> MALSTATKAATDALAANRAPTSVNAQEVHRWLQSFN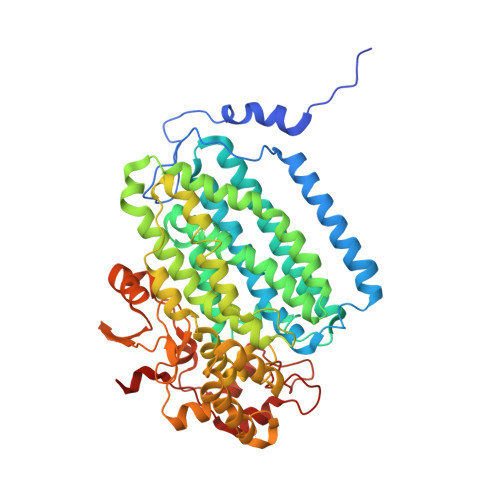WDFKNNRTKYATKYKMANETKEQFKLIAKEYARMEAVKDERQFGSLQDALTRLNAGVRVHPKWNETMKVVSNFLEVGEYNAIAATGMLWDSAQAAEQKNGYLAQVLDEIRHTHQCAYVNYYFAKNGQDPAGHNDARRTRTIGPLWKGMKRVFSDGFISGDAVECSLNLQLVGEACFTNPLIVAVTEWAAANGDEITPTVFLSIETDELRHMANGYQTVVSIANDPASAKYLNTDLNNAFWTQQKYFTPVLGMLFEYGSKFKVEPWVKTWNRWVYEDWGGIWIGRLGKYGVESPRSLKDAKQDAYWAHHDLYLLAYALWPTGFFRLALPDQEEMEWFEANYPGWYDHYGKIYEEWRARGCEDPSSGFIPLMWFIENNHPIYIDRVSQVPFCPSLAKGASTLRVHEYNGQMHTFSDQWGERMWLAEPERYECQNIFEQYEGRELSEVIAELHGLRSDGKTLIAQPHVRGDKLWTLDDIKRLNCVFKNPVKAFN>VSFRQKRTRIPLLAMTVTALAAAVCGVTTAPAATGAEVAVPLSVGAAAGNATPIPGYVIQSSAQVSDDSAVSKPGFPTSGWYPVSSRSTVYAGLLQNGKYADPFYSTNMQNVPAAQFSVPWWYRTDLNVDDTSSRTYLDFSGVLSKADVWVNGTKVATKDQVNGAYTRHDLDITAQVHTGVNSVAFKVYPNDPNRDLSMGWIDWAQTPPDQNMGIVRDVLVRRSGAVALRSAHVIQKLNSALDHADLTVKADVRNDSANAVQTTVAGTVAGKPISQTVSLAAKERKTVTFPLVGLDRPNVWWPAGMGGQHRYDLDLTASVGGTPSDAAKSKFGVRDVKATLNSSGGRQYSVNGKPLLIRGGGYTPDLFLRWNETAAADKLKYVLNLGLNTVRLEGHIEPDEFFDIADDLGVLTMPGWECCDKWEGQVNGEEKGEPWVESDYPIAKASMFSEAERLRDHPSVISFHIGSDFAPDRRIEQGYLDAMKAADFLLPVIPAASARPSPITGASGMKMNGPYDYVPPVYWYDKSQKDRGGAWSFNSATSAGVDIPTMDTLKRMMSASELDTMWKNPSAKQYHRSSSDTFGNLKLFGDALTKRYGASANLNDFVRKAQLSQYENVRAEFESHSRNYTDSTNPSTGLIYWMLNSPWTSLHWQLFDAYMDQNGAYYGAKKANEPLHIQYSHDNRSVVVINQTSNAVSGLTATTKLYNLDGTEKYSNTKTGLSVGALGAKATAVTVPAVSGLSTTYLAKNVLTDSSGKEVSRNVYWLSTKADTLNWGGSDWYYTPQSAFADLSGLNNLGQSAVGATANSVAGADGTTTTTVTLKNTSGGRLPAFYVDSKVVDSAGKPVLPVEWNDNAVSLWPGETTTLTAKYRT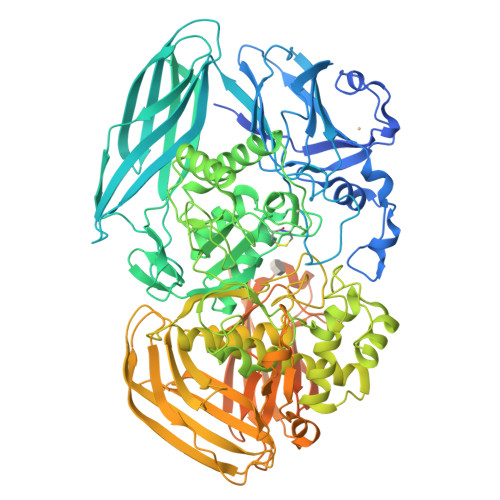ADLKGSKPSVRISGWNTGTQTVPADGSGPGPSDPVDYQAEDATIVQGAVESNHAGYTGTGFVNYDNVAGSSVEWTVTVPSAGTYDVVVRYANGTTTSRPLDFSVNGSISASGVAFGSTGTWPAWTTKTVRVTLAAGVNKIKAVATTANGGPNVDKITL[2x]> NPN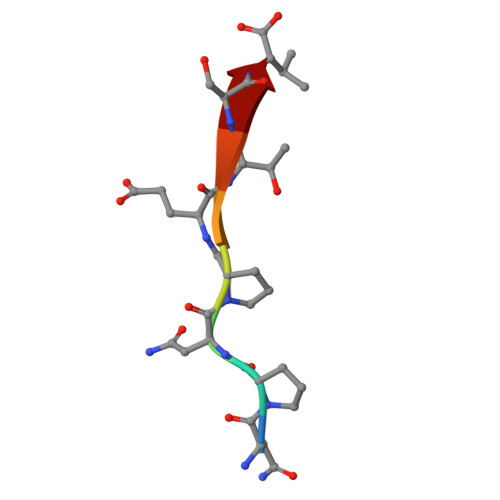PETSV> MHHHHHHHDGTENPIHDRTSDYHKYLKVKQGDSDLFKLTVSDKRYIWYNPDPKERDSYECGEIVSETSDSFTFKTVDGQDRQVKKDDANQRNPIKFDGVEDMSELSYLNEPAVFHNLRVRYNQDLIYTYSGLFLVAVNPFKRIPIYTQEMVDIFKGRRRNEVAPHIFAISDVAYRSMLDDRQNQSLLITGESGAGKTENTKKVIQYLASVAGRNQANGSGVLEQQILQANPILEAFGNAKTTRNNNSSRFGKFIEIQFNSAGFISGASIQSYLLEKSRVVFQSETERNYHIFYQLLAGATAEEKKALHLAGPESFNYLNQSGCVDIKGVSDSEEFKITRQAMDIVGFSQEEQMSIFKIIAGILHLGNIKFEKGAGEGAVLKDKTALNAASTVFGVNPSVLEKALMEPRILAGRDLVAQHLNVEKSSSSRDALVKALYGRLFLWLVKKINNVLCQERKAYFIGVLDISGFEIFKVNSFEQLCINYTNEKLQQFFNHHMFKLEQEEYLKEKINWTFIDFGLDSQATIDLIDGRQPPGILALLDEQSVFPNATDNTLITKLHSHFSKKNAKYEEPRFSKTEFGVTHYAGQVMYEIQDWLEKNKDPLQQDLELCFKDSSDNVVTKLFNDPNIASRAKKGANFITVAAQYKEQLASLMATLEAANPHFVRCIIPNNKQLPAKLEDKVVLDQLRCNGVLEGIRITRKGFPNRIIYADFVKRYYLLAPNVPRDAEDSQKATDAVLKHLNIDPEQYRFGITKIFFRAGQLARIEEAREQRLESNEPPMDFDDDIPF

The ATP-driven mutual interplay between myosin and actin drives muscle contraction and many other forms of cellular motility, including cytokinesis and directional cargo transport; yet, our molecular understanding of how these two cytoskeletal proteins communicate with each to generate force still remains incomplete. With the aid of mutant analyses based on kinetic investigations and simulations, we identified the W-helix as an important hub coupling the structural changes of switch elements during ATP hydrolysis to temporally controlled interactions with actin that are passed to the central transducer and converter. A critical role in controlling the sequence of events associated with force production appears to be played by the W-helix, which we propose to act as kind of communication zone in the inner myosin core for coupling conformational rearrangements upon nucleotide binding to cleft closure-induced β-sheet distortions by putting a stress on β1 to β3 of the central transducer; this is important to temporally couple weak-to-strong actin-binding transitions to the initiation of the power stroke and release of hydrolysis products. To gain mechanistic insights into the proposed role of the W-helix/transducer region in mediating actin binding to product release, we followed a mutational approach and replaced the two hotspot threonines in the W-loop of the myosin-2 motor domain from D. discoideum by either two alanines (AA) or three glycines (GGG) in order to reduce the rigidity of that region during weak-to-strong transition without dramatically disturbing the fold of the protein.

We crystallized the motor domains of the mutant myosins M765AA and M765GGG in complex with ADP∙VO32− and solved the atomic structures of the proteins to a resolution of 2.60 Å and 2.55 Å, respectively. The superimposed structures reveal that the mutants crystallized in the pre-power-stroke state adopting the same overall conformation as previously reported for the wildtype. Characteristic features of this pre-power-stroke state are the partially open actin-binding cleft, the up position of the converter, and the relay helix in a bent conformation. The active site elements, switch-1 and switch-2, adopt the characteristic closed conformations and coordinate the nucleotide together with the P-loop. The nucleotide position and nucleotide-binding pocket are conserved between wild-type and mutants. Only minor structural deviations from the wild-type conformation can be observed for the mutants concerning the β3, β5, and β7 strands of the central transducer, which are slightly shifted, as well as the relay helix conformation.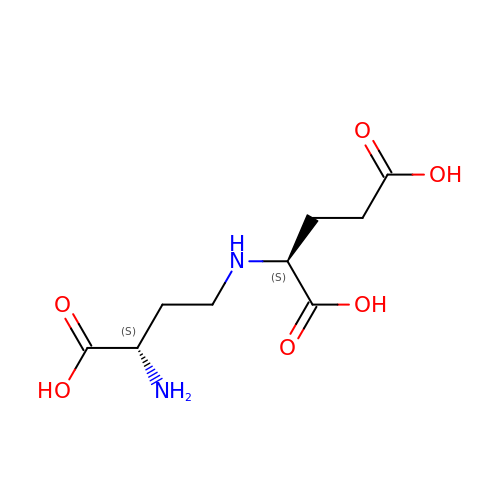N-[(3S)-3-amino-3-carboxypropyl]-L-glutamic acid | C9 H16 N2 O6 | VTEXNADNTYNYRI-WDSKDSINSA-N> RLYRADSRPPDE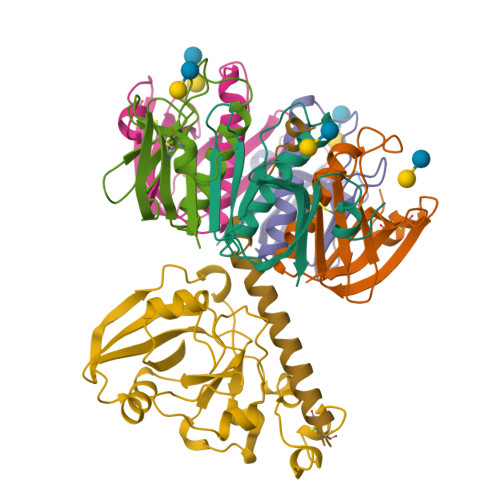IKRSGGLMPRGHNEYFDRGTQMNINLYDHARGTQTGFVRYDDGYVSTSLSLRSAHLAGQSILSGYSTYYIYVIATAPNMFNVNDVLGVYSPHPYEQEVSALGGIPYSQIYGWYRVNFGVIDERLHRNREYRDRYYRNLNIAPAEDGYRLAGFPPDHQAWREEPWIHHAPQGCG;> GDTCNEETQNLSTIYLREYQSKVKRQIFSDYQSEVDIYNRI;>[5x]APQTITELCSEYRNTQIYTINDKILSYTESMAGKREMVIITFKSGETFQVEVPGSQHIDSQKKAIERMKDTLRITYLTETKIDKLCVWNNKTPNSIAAISMKN>MNLPTAQEVQGLMARYIELVDVGDIEAIVQMYADDA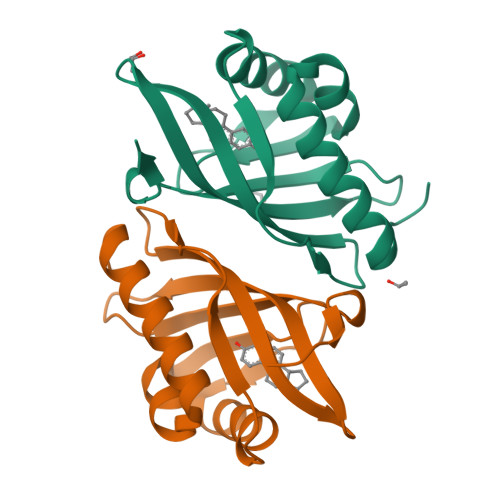TVENPFGQPPIHGREQIAAFYRQGLGGGKVRACLTGPVRASHNGCGAMPFRVEMVWNGQPCALDVINVMRFDEHGRIQTMQAYWSEVNLSVREPQ[2x]> MGEDVIDSLQLNELLNAGEYKIGELTFQSIRSSQELQKKNTIVNLFGIVKDFTPSRQSLHGTKDWVTTVYLWDPTCDTSSIGLQIHLFSKQGNDLPVIKQVGQPLLLHQITLRSYRDRTQGLSKDQFRYALWPDFSSNSKDTLCPQPMPRLMKTGDKEEQFALLLNKIWDEQTNKHKNGELLSTSSARQNQTGLSYPSVSFSLLSQITPHQRCSFYAQVIKTWYSDKNFTLYVTDYTENELFFPMSPYTSSSRWRGPFGRFSIRCILWDEHDFYCRNYIKEGDYVVMKNVRTKIDHLGYLECILHGDSAKRYNMSIEKVDSEEPELNEIKSRKRLYVQN

The conserved shelterin complex caps chromosome ends to protect telomeres and regulate telomere replication. In fission yeast Schizosaccharomyces pombe, shelterin consists of telomeric single- and double-stranded DNA-binding modules Pot1-Tpz1 and Taz1-Rap1 connected by Poz1, and a specific component Ccq1. Here, we report the crystal structures of Pot1DBD-single-stranded-DNA, Pot1372-555-Tpz1185-212 and Tpz1425-470-Ccq1123-439 complexes and propose an integrated model depicting the assembly mechanism of the shelterin complex at telomeres. Overall, our findings provide valuable structural information regarding interactions within fission yeast shelterin complex at 3’ ss telomeric overhang.

Next, we crystallized Pot1DBD in complex with Tel18 and determined the complex structure by molecular replacement at a resolution of 3.0 Å. The calculated electron density map allowed us to unambiguously trace most of the complex except for a disordered loop between Pot1OB1 and Pot1OB2 (residues 174–198). The overall structure of the Pot1DBD-Tel18 complex reveals that Pot1OB1 and Pot1OB2 pack in tandem to adopt an elongated conformation, and the ssDNA-binding grooves of the two OB folds are connected with a kink at the OB1-OB2 interface. The telomeric ssDNA Tel18 meanders along a long continuous groove on the surface of Pot1DBD in an ‘S’-shaped conformation with its backbone exposed to solvent and its bases partially or completely buried in a solvent-excluded contact area of ~1,900 Å2. Close inspection of the Pot1DBD-Tel18 interface reveals that G1-C6 and G10-T18 are respectively recognized by Pot1OB1 and Pot1OB2 almost in the same manner as in the Pot1OB1-Tel6 and Pot1OB2-Tel9 subcomplexes whose structures were previously determined. In the Pot1DBD-Tel18 complex, the Pot1OB1 moiety recognizes G2T3T4 with high specificity, defining the binding register of the first telomere repeat (G1-C6). Compared with Pot1OB1, Pot1OB2 confers only moderate sequence specificity for nucleotides G11, G16 and T18. Trinucleotide linker A7G8G9 in Tel18 is the most frequently occurring linker sequence in S. pombe telomeres. This short nucleotide linker adopts a highly zigzagged conformation and is sandwiched between the two OB folds, with the bases of G8 and G9 stacking together on the plane formed by G10 and the side chain of His305 from Pot1OB2. Here, we consider that the structurally separable Pot1OB1 and Pot1OB2 together with the long flexible loop between them endow S. pombe Pot1DBD with more flexibility capable of binding degenerate telomeric sequences.>[6x]MAMAQELTAMSAWVNQDGSTLYINSIN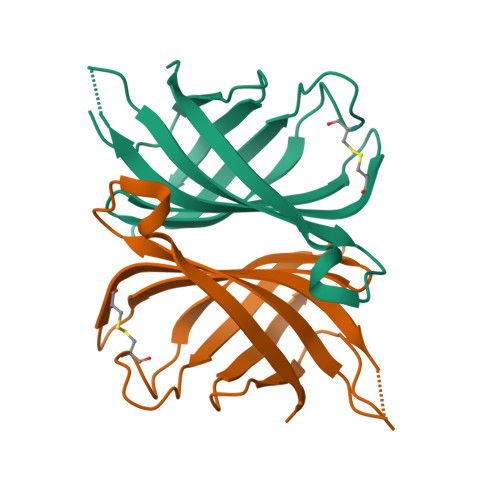AQGELTGSYINRAAGFACQNSPYPVNGWVFGTAISFSTKWLNSVESCNSITSWSGFYINTGGQGKISTLWQLVVNGSSSPSQILKGQDVFSQTSA> MGHHHHHHMSHIIN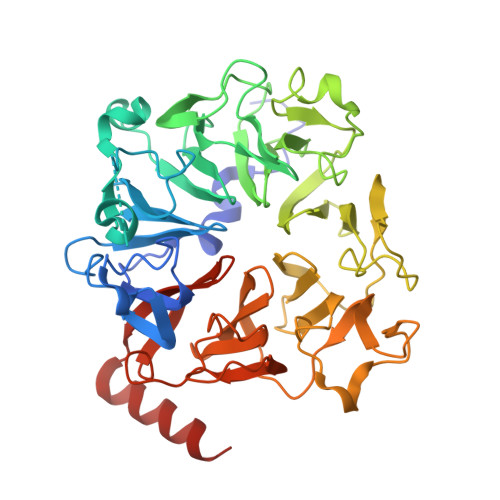AQEDYKHMYLSVQPLDIFCWGTGSMCELGLGPLAKNKEVKRPRLNPFLPRDEAKIISFAVGGMHTLALDEESNVWSWGCNDVGALGRDTSNAKEQLKDMDADDSSDDEDGDLNELESTPAKIPRESFPPLAEGHKVVQLAATDNMSCALFSNGEVYAWGTFRCNEGILGFYQDKIKIQKTPWKVPTFSKYNIVQLAPGKDHILFLDEEGMVFAWGNGQQNQLGRKVMERFRLKTLDPRPFGLRHVKYIASGENHCFALTKDNKLVSWGLNQFGQCGVSEDVEDGALVTKPKRLALPDNVVIRSIAAGEHHSLILSQDGDLYSCGRLDMFEVGIPKDNLPEYTYKDVHGKARAVPLPTKLNNVPKFKSVAAGSHHSVAVAQNGIAYSWGFGETYAVGLGPFEDDTEVPTRIKNTATQDHNIILVGCGGQFSVSGGVKLSDEDAEKRADEMDDLEHHHHHH>MCGRFLRRLLAEESGRSTPVGRLLLPVLLGFRLVLLAASGPGVYGDEQSEFVCHTQQPGCKAACFDAFHPLSPLRFWVFQVILVAVPSALYMGFTLYHVIWHWELSGKGKEEETLIQGREGNTDVPGAGSLRLLWAYVAQLGARLVLEGAALGLQYHLYGFQMPSSFACRREPCLGSITCNLSRPSEKTIFLKTMFGVSGFCLLFTFLELVLLGLGRWWRTWKHKSSSSKYFLTSESTRRH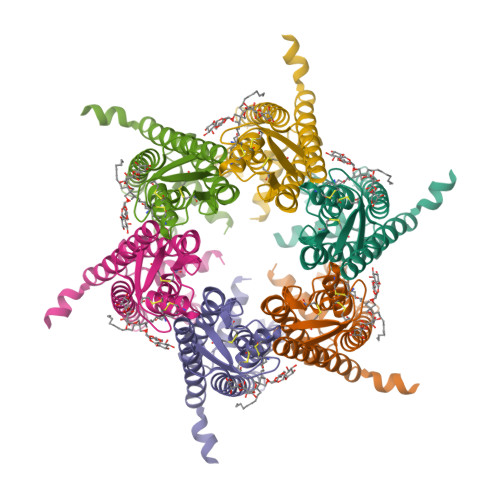KKATDSLPVVETKEQFQEAVPGRSLAQEKQRPVGPRDA[6x]>[4x]MTQGAVKTTGKRSRAVSAKKKAILSAALDT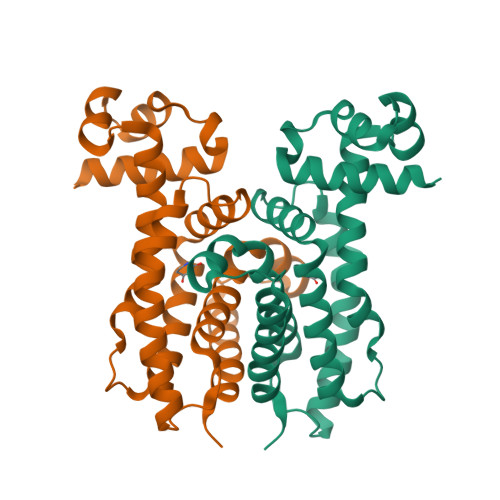FSQFGFHGTRLEQIAELAGVSKTNLLYYFPSKEALYIAVLRQILDIWLAPLKAFREDFAPLAAIKEYIRLKLEVSRDYPQASRLFCMEMLAGAPLLMDELTGDLKALIDEKSALIAGWVKSGKLAPIDPQHLIFMIWASTQHYADFAPQVEAVTGATLRDEVFFNQTVENVQRIIIEGIRPR> MNKQIFVLYFNIFLIFLGIGLVIPVLPVYLKDLGLTGSDLGLLVAAFALSQMIISPFGGTLADKLGKKLIICIGLILFSVSEFMFAVGHNFSVLMLSRVIGGMSAGMVMPGVTGLIADISPSHQKAKNFGYMSAIINSGFILGPGIGGFMAEVSHRMPFYFAGALGILAFIMSIVLIHDPKKSTTSGFQKLEPQLLTKINWKVFITPVILTLVLSFGLSAFQTLYSLYTADKVNYSPKDISIAITGGGIFGALFQIYFFDKFMKYFSELTFIA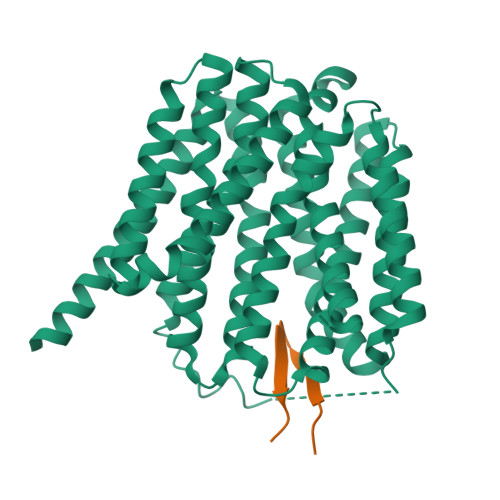WSLLYSVVVLILLVFANDYWSIMLISFVVFIGFDMIRPAITNYFSNIAGERQGFAGGLNSTFTSMGNFIGPLIAGALFDVHIEAPIYMAIGVSLAGVVIVLIEKQHRAKLKEQNMENLYFQGKLGPEQKLISEEDLNSAVDHHHHHHHHHH;> SVENHWYYFYWYMSP(3-ethoxythiophen-2-yl){4-[4-nitro-3-(pyrrolidin-1-yl)phenyl]piperazin-1-yl}methanone | C21 H26 N4 O4 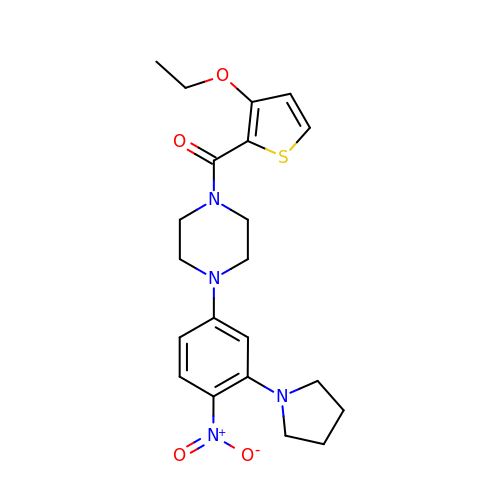S | LAYJOGOQGVGOCO-UHFFFAOYSA-N> MGAQVTRQQTGTHENANIATNGSHITYNQINFYKDSYAASASKQDFSQDPSKFTEPVVEGLK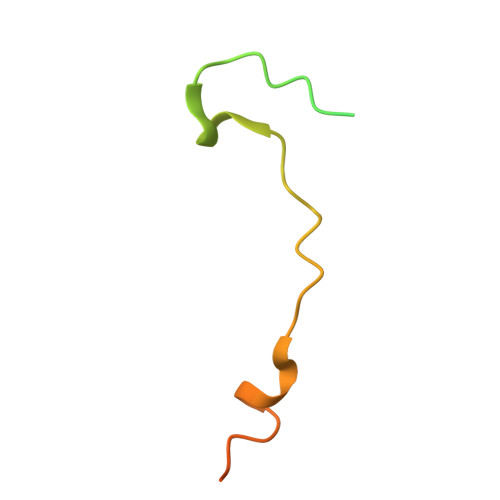AGAPVLK>MAHHHHHHMSIEDLARANVRALTPYQSARRLGGKGDVWLNANEFPTAVAFQLTEQTLNRYPEPQPKAVIESYARYAEVKPEQVLVSRGADEGIELLIRAFCEPGEDAVLYCPPTYGMYSVSAETIGVECRTVPTLADWQLDLPGIEARLDGVKVVFVCSPNNPTGQIIDPQSMRDLLEMTRGKAIVVADEAYIEFCPQATLAGWLSDYPHLVVLRTLSKAFALAGLRCGFTLANAEVINVLLKVIAPYPLSTPVADIAAQALSPEGIAAMRQRVAQILDERRYLVEQLRGIACVEQVFDSETNYVLARITASSAVFKSLWDQGIILRDQNKQPSLSGCLRITIGTRAESQRVIDALTAENV[4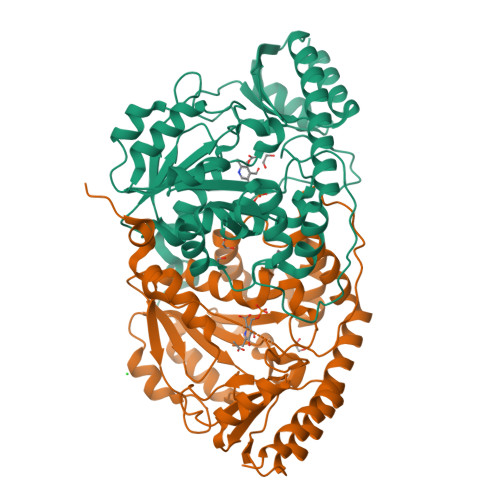x]>[3x]GLFDAPGRSQFVPADQA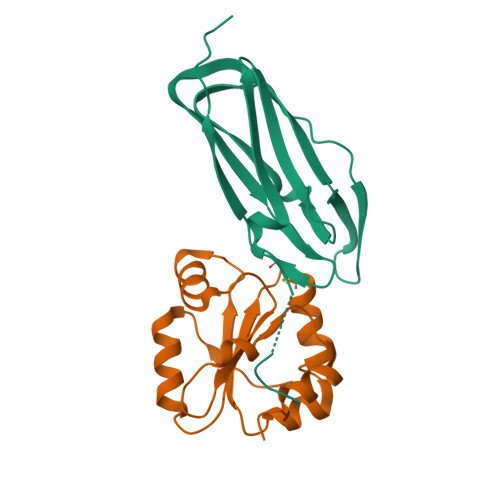FAFDFQQNQHDLNLTWQIKDGYYLYRKQIRITPEHAKIADVQLPQGVWHEDEFYGKSEIYRDRLTLPVTINQASAGATLTVTYQGSADAGFCYPPETKTVPLSEVVANNAAPQPVSVPQQEQPTAQ;>[3x]ATHTAQTQTHLNFTQIKTVDELNQALVEAKGKPVMLDLYADWCVASKEFEKYTFSDPQVQKALADTVLLQANVTANDAQDVALLKHLNVLGLPTILFFDGQGQEHPQARVTGFMDAETFSAHLRDRQPHHHHHH>[2x]GCGGAUUUAGCUCAGUUGGGAGAGCGCCAGACUGAAGAUCUGGAGGUCCUGUGUU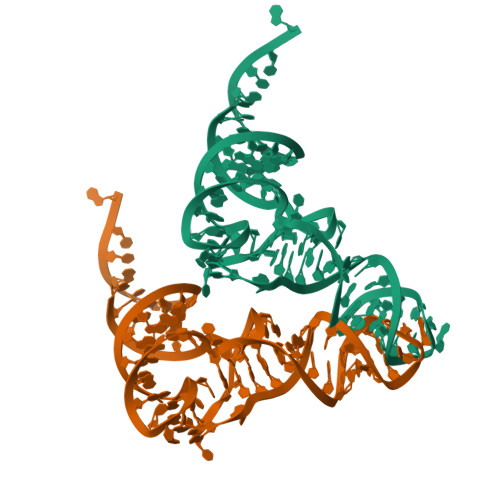CGAUCCACAGAAUUCGCACCA>MTRQMILAVGQQGPIARAETREQVVGRLLDMLTNAASRGVNFIVFPELALTTFFPRWHFTDEAELDSFYETEMPGPVVRPLFETAAELGIGFNLGYAELVVEGGVKRRFNTSILVDKSGKIVGKYRKIHLPGHKEYEAYRPFQHLEKRYFEPG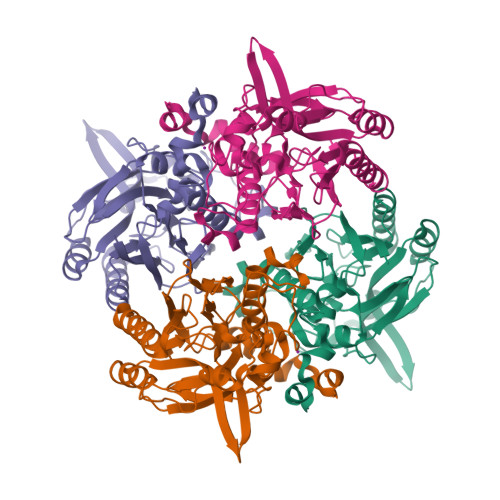DLGFPVYDVDAAKMGMFICNDRRWPETWRVMGLKGAEIICGGYNTPTHNPPVPQHDHLTSFHHLLSMQAGSYQNGAWSAAAGKVGMEEGCMLLGHSCIVAPTGEIVALTTTLEDEVITAALDLDRCRELREHIFNFKAHRQPQHYGLIAEF[4x]>[20x]MGNVQTSVNTYNITGDGNSFTPTSDMTSTAAPAIDLKPGVLNPTGKLWRPVGTSVATIDSLAIVSDRFGQYSFVNEGMRETFSKALFDINMWQPLFQATKTGCGPIVLSSFTTTTSGYVGATAGDALDNPVTNGVFISTVQIMNLQRTIAARMRDVALWQKHLDTAMTMLTPDISAGSASCNWKSLLAFAKDILPLDNLCLTYPNEFYNVAIHRYPALKPGNPDTKLPDAQAHPLGEVAGAFNAATSEVGSLVGSSSTLSQAISTMAGKDLDLIEADTPLPVSVFTPSLAPRSYRPAFIKPEDAKWIAEFNNSSLIRKTLTYSGATYTVQLGPGPTRVIDMNAMIDSVLTLDVSGTILPYDTNPDLSTSVPAFVLIQTSVPIQQVTTAANITAITVVSAAGASAINLAINVRGQPRFNMLHLQATFERETITGIPYIYGLGTFLIPSPTSSSNFSNPTLMDGLLTVTPVLLRETTYKGEVVDAIVPATVMANQTSEEVASALANDAIVLVSNHLNKLANVVGDAIPVASRTDDSATSAIVSRLAVQHKLSQVGQASPTPPDYPLLWRRAKRAASMFVSNPSLALQVGIPVLTQSGMLSALTSGVGTALRTGSLGKGVTDASEKLRARQSLTVAKQAFFDQIGSLWPGK;>MAQRQFFGLTYNFYGQPAPLFDLNDLQELAGCYARPWTSRFSHLAISTGSLPVWSARYPSVASRNIVVNTLLGAHLNPFAGGQITSHQGITWRDPVLSSLAPVPAIQPPPVWAVAENVLLDSNNYPTYVLNLSSMWPINQDVHIMTMWALSDQGPIYHLEVPVDPMPAATTAALMAYTGVPIAHLAQTAYRFAGQLPQSPDSTMVSTIRWLSAIWFGSLTGRLNRSRTCNGFYFEFAKPALNPDQAVLKWNDGARAAPPAAAQSSYIRCISPHWQHQIVEVAGALMSQSVTAVTGLPALIDEATLPAWSQGVANLTGNGQGVVPCLDYNPVPMAAARHLQWRQDGLITAAQEAQLNNDYTAYALTIERHLTAMLVANPIAAGRMPIQPFNAADFGQAGQTAAAVALAQAMFV[2x];> MAAVFGIQLVPKLNTSTTRRTFLPLRFDLLLDRLQSTNLHGVLYRALDFNPVDRSATVIQTYPPLNAWSPHHAFIENPLDYRDWTEFIHDRALAFVGVLTQRYPLTQNAQRYTNPLVLGAAFGDFLNARSIDIFLDRLFYDPTQDSPITAITKFPYQWTIDSNVTTDSVRTSAGCKYITLYGYDPSRPSTPATYGKHRPTYATVFYYSTLPARSRLLANLAAGPTVLEHFDSPTYGPHLLLPQTGDVLGYSSSLISQAALLMVESVMDALRDNANASASTAVTRLDQSYHPVTSFDPSTFNTLLQRATNLALLAVQGVQSESAIPAIPTMSDVRSFVARLMAEGDPQQWFPYRVDQILYWPESPFVPPIGPFYAPFRPVNFPFTTGSYTVVPDASRPLRLLPQYRNATITVQQADDAYEDTALSPLITTHGFCVTGGVFTSIYDISGDPTAYPPAQLVDAPNDYFDRERMARRDLFRRLRAPADRSAIKDRAVFDFLASLVNPTTANPVLDTSFSMAYLGASSAHANADEPVILADIRSGSIPGL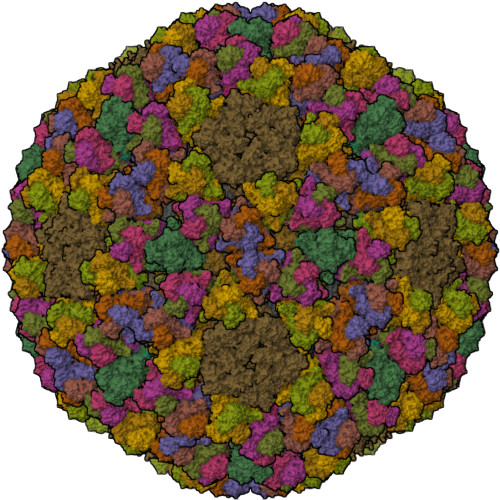PIPRRIVQFGYDVVHGSLLDLSRAVPTGTFGLVYADLDQVEDAGTDMPAANRAAIAMLGTALQMTTAGGVSVLKVNFPTRAFWTQVFNLYATHATTLHLVKPTIVNSSEVFLVFGGRQSNGALRSTTALQRALLSLYARNAAIDRAVTHIPFFGVPDDGTSDLGIDAVRLFDPMFSDAVANLPSNALASLVSRVVPSSIMFTRVPSNGPVSTTIYGKRTFLSNRRRARLRDVPMLITTTLVHQRRFTTPPTFTLFSSEAVPVTTLVAAGYNSFISEQTRNPNLAHLLDLGTGPECRILSLIPPTLQVTMSDSRPCAELMASFDPALTAYVQGDYSTAAFWNGIRCDSATAIFTIGAAAAAAGTDLIAFVQQLIPRIVAAGGTRMWLQLNTPLYEVSSLPDLIEIDLRDHVYRFNGGERVEPYADPVPLQQAIAALLPAAALSWHTLSPTCDWLPYIIGVGSPLNLSDINTAISYSRLTPILHIDTTTPPLRVNPVPTPLNQQCAIRITSLDPAAVLSVQHNGVEVIGGTPGNVISVAGAAALQYILANQEFLLQFTPTLPGIFDVFLTTLGQPPVPRGSFTITPPPTTVALNMPPPRQLDFTDVGNDARITCDPYYQLAVCIFKDGQYVRVNPEKASVVTNAPNRDLHFVLDLADNHVLLYLCDVTPSGLGDRIAFPIVDIYRIAFPRNTPVRASLPYTGGGAHLTSGGNPFMSLTTPPAVLPAGVALAALSTSVATQYPTYTLPAGVYEYVIE;>[2x]MPRRSARKAQSAIASPADTNVVPAKDAPTTNSPPSTTSPNQAAADANQQQAGIVSSQSGPNAVGDSAPSSSVNNDGDIITRPTSDSIAAVANATKPAAVVSDPQSMKVTPIVNPSSYVCNVCNARFSTMSALSEHLRSDHRDDASTLLATPMINNAIRSFLTAWDDIRILSPDVSSKSLSAYLDSAVANGPELIIEDTGLCTSFMLLDNIPSAHLTKELIGFTWFMQMYQMTPPLPEGAVNRIVCMTNWASLGDEGRGLEVRLPPPTDSSVHAYKTVLSRGYIDNAQFNPLALRSNVLLMLLQFTLSNLKINKSSTFTSDVTTITSGRMIRAFEGRPELLALAYPGRAVLPTQTKNAQFLSTAIADRIGRLDRANLIGGEVSAMVECMELCDALTLHIRETYIMLLRSMHQDPTQIVQIVNECANNLLNSTIPISLRPTILCPWFASSEDLRLQQVMHLVNISSNTAAALPLVEALSTLLRSVTPLVLDPTVLTNAITTISESTTQTISPISEILRLLQPMGNDYAAFWKCIASWAYNGLVTTVLSEDAFPDSSQSITHLPSMWKCLFLTLAGPMTSDPHSPVKVFMALANLLAQPEPIAIGVPGMHQTTPASQFSHPGVWPPGFLNPQLINPQQAPLLRAFAEHIRANWPQPSEFGYGSTLQGSANLFIPSNRMVYPWPNQPLPRLTVAPTYDSAMSNWISTTIAFFIRVVNSVNMTATVNDLTRRTMTGVMTAMRQVKTMTPFYIQHMCPTELSVLASVTVTPPFQVPFTRLVQNDVITNVLVARVDPAQRGDAAVDIRATHATFAAALPVDPAAIVVAMLCGQTETNLIPSHHYGKAFAPLFASNAMFTRNQRAVITREAFVCARSAVAQCQDAGFLVPRPLDALRQFDVTSAAAAEIMHAVNDAFKTAFDLDGALLDGLALYGDPRIADLSAAYLQYGGNVVREHVPPGPSHIHRALQQVESTFMAEMNLFNVARGNLYLVQTATNGNWSPMAPVAAPPFVRGGPNVRVVGRFGTIVPRPNGLEPQLIDDGNVPRDIAGDWVYPSDVLQVSVAVFRDYVWPMVKAGRTRVLVELGHYVYTLHYYDPQISLDEAPILEEWLSKINPAGIPPVPFCIPIPQVYPCITARRVHYAFTSENNNDSLFSTNAASIDTAFGENAAVSPLRWPGLVDPNYRVGTNDLPNRITLYNSLYRYNFTYPTLDGIMYVRSAT> MGKKLSLIDFNEIYNEENLITRANPIENHEFSDDG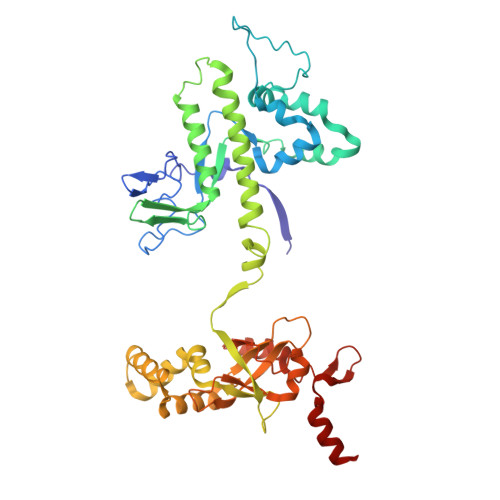IYSERIFGSYNEDDDDKDIDTIGWINIEPYYIINPILFTIIKKCIPSINKIINYQQSIDQNGENIDLTEEIGEDDYIGLVKFKDNFDDLLEKYTDKKKYQKEYDFLIENHDKIFINKLPVFSHKLRPATLLTGSKGKVLAFDEINNYYNFVIEYINQINEGVVSDDSIDLLLLPLLYNMQFYANNILTRIISEYLRGKKGFLRKNIMGSRINFSARNVITPLIGHPIDEVAMPYKTFAELYKFQLINLISKVKGINYNEALKFWEKGILGFNQELYNYMEELITKTKGGCTFLLNRNPTISIGSILYLKIGLIKKDYKDLTLGISNNLLSALSGDYDGDVLNIIPVFDNKMKEHFSLLSPQNFLVDRNNGRFNGDFDLQKDQILGIFILNN> HHHHHHMQHLVLIGFMGSGKSSLAQELGLALKLEVLDTDMIISERVGLSVREIFEELGEDNFAMFEKNLIDELKTLKTPHVISTGGGIVMHENLKGLGTTFYLKMDFETLIKRLNQKEREKRPLLNNLTQAKELFEKRQALYEKNASFIIDARGGLNNSLKQVLQFIA

SK catalyzes the specific phosphorylation of the 3-hydroxyl group of shikimic acid, using ATP as a co-substrate. The shikimate pathway is comprised of seven enzymatic components that convert erythrose 4-phosphate and phosphoenolpyruvate into chorismate, for subsequent synthesis of aromatic compounds. SKs belong to a class of P-loop kinases that share a homologous α-β-α fold. Overall, these structures have a characteristic α-β-α fold that consists of the CORE domain (residues 1–31, 61–108, and 124–162), the SB domain (residues 32–60), and the LID region (residues 109–123) in the monomer.

We also determined the structure of mutant R57A that lacked enzyme activity. Enzymatic analysis of R57A, R116A and R132A revealed that these mutants completely lost enzyme activity, suggesting that R57 and R132, from the CX site, are important in catalysis. In the wild-type HpSK, the guanidino group of R57 forms hydrogen bonds with the two carboxyl groups from E53 and E60. Replacement of the guanidino side chain with a methyl group at this pocket eliminates these interactions in R57A. Instead, E53 from the SB domain forms hydrogen bonds to the guanidino group from R132 (E53 [Oε1]-R132 [Nη1]: 2.21 Å; E53 [Oε2]-R132 [Nη2]: 3.58 Å) located at α6 (CORE). The E53–R132 proximity in R57A appears to induce a conformational move for the SB domain (residues 43–63; α3, the α3–α4 loop, and α4) and slightly influences the CORE domain. The R57A mutant structure shows a notable shift of the SB domain owing to the interactions between E53 and R132, rather than those between E53 and R57 in the wild-type structure, revealing a crucial role for R57 and R132 in defining the best active-site geometry to accommodate promising substrates.>[3x]EQEMVQVFIPAQAVGAIIGKKGQHIKQLSRF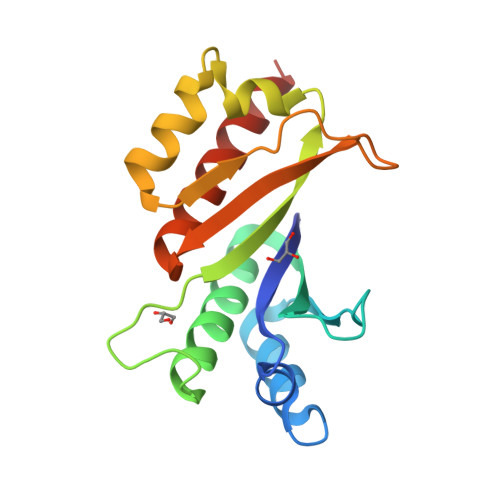ASASIKIAPPETPDSKVRMVIITGPPEAQFKAQGRIYGKLKEENFFGPKEEVKLETHIRVPASAAGRVIGKGGKTVNELQNLTAAEVVVPRDQTPDENDQVIVKIIGHFYASQMAQRKIRDILAQVKQQHQK>MSKATYKERAATHPSPVAAKLFNIMHEKQTNLCASLDVRTTKELLELVEALGPKICLLKTHVDILTDFSMEGTVKPLKALSAKYNFLLF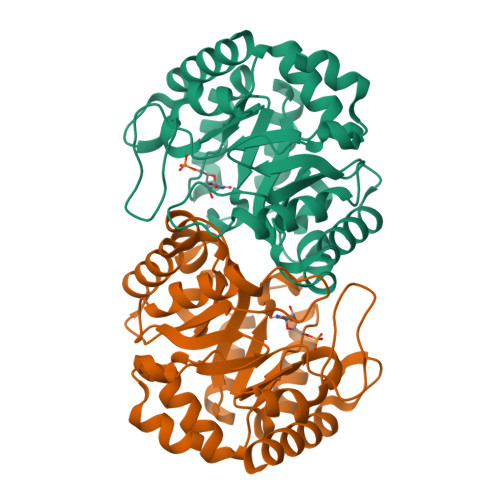EDRKFADIGNTVKLQYSAGVYRIAEWADITNAHGVVGPGIVSGLKQAAEEVTKEPRGLLMLAELSCKGSLATGEYTKGTVDIAKSDKDFVIGFIAQRDMGGRDEGYDWLIMTPGVGLDDKGDALGQQYRTVDDVVSTGSDIIIVGRGLFAKGRDAKVEGERYRKAGWEAYLRRCGQQN[2x]GEN1 belongs to the Rad2/XPG family of structure-selective nucleases that are conserved from yeast to humans. Although the catalytic cores are well conserved in the superfamily, substrate recognition is highly diverse: XPG/Rad2/ERCC5 recognizes bubble/loop structures during nucleotide-excision repair (NER), FEN1 cleaves flap substrates during Okazaki fragment processing in DNA replication, EXO1 is a 5'->3' exonuclease that is involved in HR and DNA mismatch repair (MMR) and GEN1 recognizes Holliday junctions. Interestingly, GEN1 shows versatile substrate recognition accommodating 5’ flaps, gaps, replication fork intermediates and Holliday junctions. According to the current model, however, the primary function of GEN1 is HJ resolution and it is suggested to be a last resort for the removal of joint molecules before cytokinesis.

In order to structurally characterize human GEN1, we crystallized the catalytically inactive variant GEN12-505 D30N, denoted GEN1 for simplicity, in complex with an immobile Holliday junction having arm lengths of 10 bp. The structure was determined experimentally and refined up to 3.0 Å resolution with an Rfree of 0.25. The HJ crystallized bridging between two protein monomers in the asymmetric unit. The overall structure of GEN1 resembles the shape of a downwards-pointing right hand with a 'thumb' extending out from the 'palm' and the DNA is packed against the ball of the thumb. The palm contains the catalytic core, which is formed by intertwined XPG-N and XPG-I domains (Figure 1A/B, green). Notably, a small globular domain (residues 390–464) was found extending the GEN1 nuclease core at the wrist (pink). The domain has a chalice-shaped structure with three antiparallel β-strands packed against a C-terminal α-helix and it forms a characteristic aromatic cage. The GEN1-HJ structure revealed that the upstream DNA-binding interface acts as a docking site for double-stranded DNA and that the chromodomain secures its position. The DNA is bound at the upstream interface and the hydrophobic wedge but does not extend into the active site or to the downstream interface (Figure 1B/C/D).

>MGVNDLWQILEPVKQHIPLRNLGGKTIAVNLSLWVCEAQTVKKMMGSVMKPHLRNLFFRISYLTQMDVKLVFVMEGEPPKLKADVISKRNQTRYGSSGKSWSQKTGRSHFKSVLRECLHMLECLGIPWVQAAGEAEAMCAYLNAGGHVDGCLTNDGDTFLYGAQTVYRNFTMNTKDPHVDCYTMSSIKSKLGLDRDALVGLAILLGCDYLPKGVPGVGKEQALKLIQILKGQSLLQRFNRWNETSCNSSPQLLVTKKLAHCSVCSHPGSPKDHERNGCRLCKSDKYCEPHDYEYCCPCEWHRTEHDRQLNEVENNIKKKACCCEGFPFHEVIQEFLLNKDKLVKVIRYQRPDLLLFQRFTLEKMEWPNHYACEKLLVLLTHYDMIERKLGSRNSNQLQPIRIVKTRIRNGVHCFEIEWEKPEHYAMEDKQHGEFALLTIEEESLFEAAYPEIVAVYQKQKLEIKGKKQKRIKPKENNLPEPDEVMSFQSHMTLKPTCEIFHKQNSL[2x]N-{[(4-nitrophenyl)carbonyl]carbamoyl}-beta-D-glucopyranosylamine | C14 H17 N3 O9 | 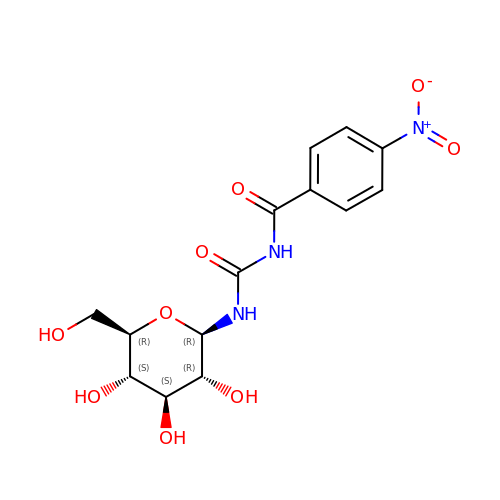TXVZHPDFTXBTMX-BZNQNGANSA-N>GIDPFTTRPSSDLTAFREHFAKAKHIAIITGAGVSAESGVPTFRGPGGFWRKWQAQDLATPEAFSRDPSLVWEFYHYRREVMRSKMPNPAHLAIAECEARLGQQGRSVVIITQNIDELHHRAGSKHVYEIHGSLFKTRCMSCGEVKANHKSPICPALDGKGAPDPNTKEARIPVELLPRC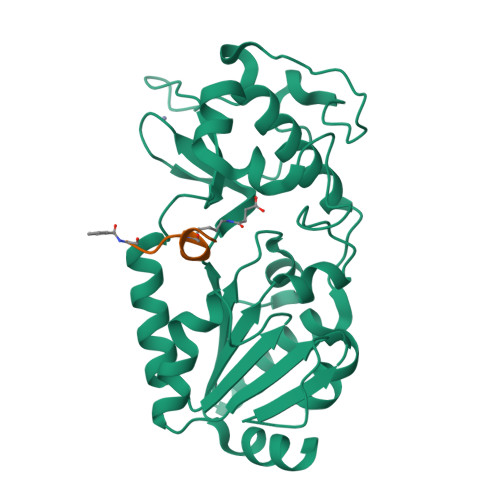ERKSCNGLLRPHVVWFGETLDSDILTAVERELEKCDLCLVVGTSSIVYPAAMFAPQVASRGVPVAEFNMECTPATQRFKYHFEGPCGSTLPPALE[2x]> DSYELSPQLEELITKVSKAHQETFPSLCQ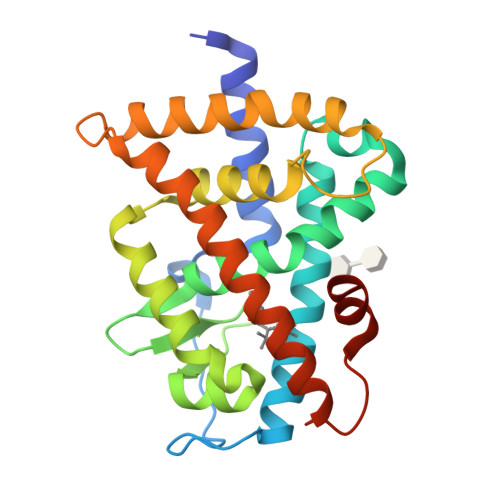LGKYTTNSSADHRVQLDLGLWDKFSELATKCIIKIVEFAKRLPGFTGLSIADQITLLKAACLDILMLRICTRYTPEQDTMTFSDGLTLNRTQMHNAGFGPLTDLVFAFAGQLLPLEMDDTETGLLSAICLICGDRMDLEEPEKVDKLQEPLLEALRLYARRRRPSQPYMFPRMLMKITDLRGISTKGAERAITLKMEIPGPMPPLIREMLENPEMFE> EKEAMNTRESGKASSSLGLQDFDLLRVIGRGSYAKVLLVRLKKTDRIYAMKVVKKELVNDDEDIDWVQTE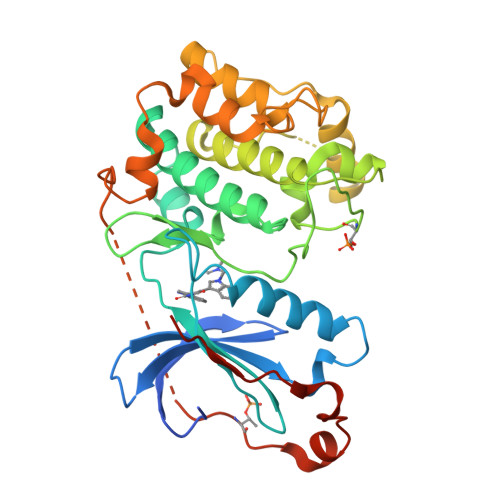KHVFEQASNHPFLVGLHSCFQTESRLFFVIEYVNGGDLMFHMQRQRKLPEEHARFYSAEISLALNYLHERGIIYRDLKLDNVLLDSEGHIKLTDYGMCKEGLRPGDTTSTFCGTPNYIAPEILRGEDYGFSVDWWALGVLMFEMMAGRSPFDIVGSSDNPDQNTEDYLFQVILEKQIRIPRSMSVKAASVLKSFLNKDPKERLGCLPQTGFADIQGHPFFRNVDWDMMEQKQVVPPFKPNISGEFGLDNFDSQFTNERVQLTPDDDDIVRKIDQSEFEGFEYINPLLMSAEECV> KMRIPNYQLSPT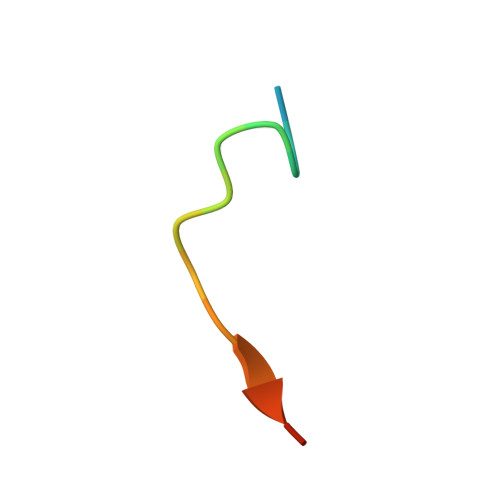KLPS>MSKIAPQCQNLREQVNQLIELLRQEPTLRSQQDTSIVETALGKALSPRFEIVFAGAFSAGKSMLINALLERELLYSAEGHATGTECHIEYANANEERVVLTFLSEAEIRQQALILAKYLNVNVGDLNINQPEAVKVVSQYCQKIIAEEGGENKSERAKQANALHLLLIGFEQNRERINTVQNSTYSMDQLNFSSLAEAAGYARRGANSAVLKRLDYFCNHSLLKDGNVLVDLPGIDAPVKEDAERAYRKIESPDTSAVICVLKPAAAGDMSAEETQLLERISKNHGIRDRVFYVFNRIDDTWYNTQLRQRLEGLIQSQFRDNSRVYKTSGLLGF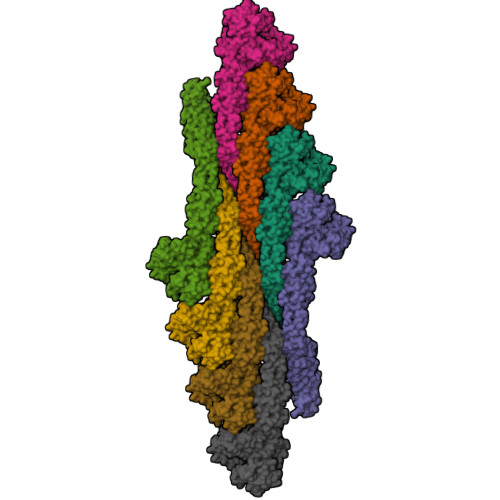YGSQVKQTNSSTRFGLDSIFATTIKGFDGEEETPQFVSEFNNYCANSGKLLSTAFRVSVNGYETSNENYVRILSEWGIPLVDQLIHDSGIESFRSGIGLYLAEEKYPELFATLANDLQPLCIALRQFYLENYRQLDSQPREIAAMKAQELTLLNQEMQNLGIEFKKYMSAQINDVVIGNDREFDQDFTKLKARMVARLDELLKTFSVMNAYKRATESHPRNSTAPFIAVLVEALYYLANELEDAFIEAIHELVKNFFQRLGDRLRKVDCYHQVYRLVGNDGGIEQLLRRAEEDITKALVNEARTECDRYVRESPRFYDEGTFSIYQFRQTLQQTSQGYDAQAIVEAEPAIKELLKLDFEPKVFNTVRKNFRQTVNNTLKTHLLPMAEEQAQIILEQYDVARKYREQTLEQDAEEKIARNSRLQSEIKQKIDLYQTSIVSINECLKAMQIFEQLPVITESDITKQAEIVADADFVEIVELEHHHHHH[8x]> MANSKNSIFVGGAGRVKQTIEGLAQSAFKPGQLLARAAGDAIDVTAKAST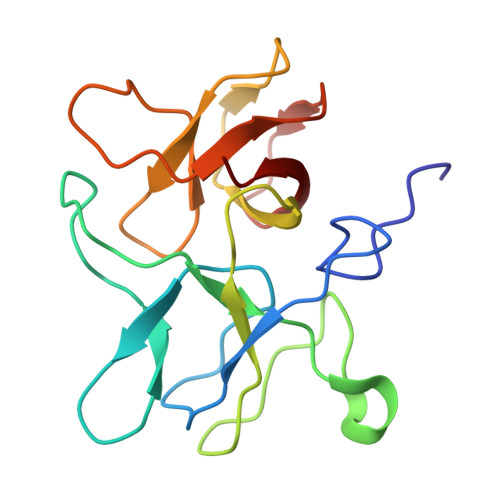TYGNEFLICDDQPQTLGGGTDVAVTAGDTVQAISVLPGQYVLLSFAATQNVTTKGAAVASNGDGNFKLGNPATEQTFAVTEEIINVTTAGTLVLCRAI>MNTFVNEFRNELETHILPFWAKLKDDENGGYYGLVDYDLHVHKDAGKGGIATCRQLWAFSAAYRVLKKEAYLQQANHAYRFLTEYVFDHQYKGLYWMVDYKGNPSDDRKHVYAQAFGVYALTEYYRVTQNQEALDYAKQLYKLIETVGFNEETNAYKEEFNRKWEEQSNEMLSENGVIADITMNTHLHVLEAYTNLYRVWEDEQLKGRIANL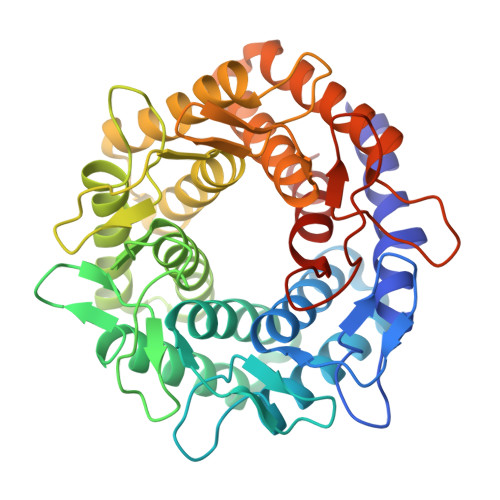IDLFYEKVFDKQSKFLQVFFNNHWESIIDLKSYGHDIEASWLIDDALKVTGNNDRKYTQMVIDIAYNIEKKGVLKDGSLAYENENGKIDYTRVWWVQVEAMVGFYNAYEKTKDEKFLKAVERIWDYVKTYMIDSREGGEWYWSVEADGQPTKREIAGPWKCPYHNARFCLEFIERVGK[2x]>MADDMERIFKRFDTNGDGKISLSELTDAL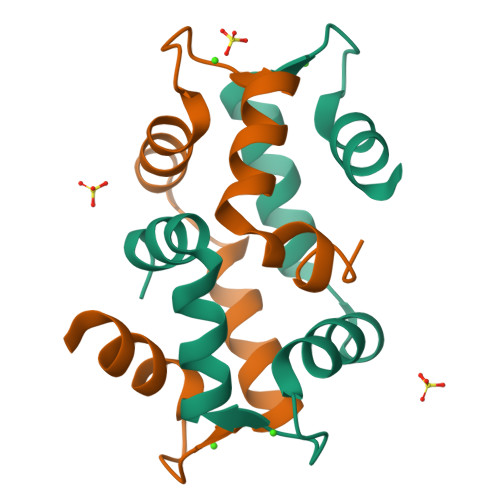RTLGSTSADEVQRMMAEIDTDGDGFIDFNEFISFCNANPGLMKDVAKVF[2x]2-AMINO-5,6-DIMERCAPTO-7-METHYL-3,7,8A,9-TETRAHYDRO-8-OXA-1,3,9,10-TETRAAZA-ANTHRACEN-4-ONE GUANOSINE DINUCLEOTIDE | C20 H24 N10 O13 P2 S2 | 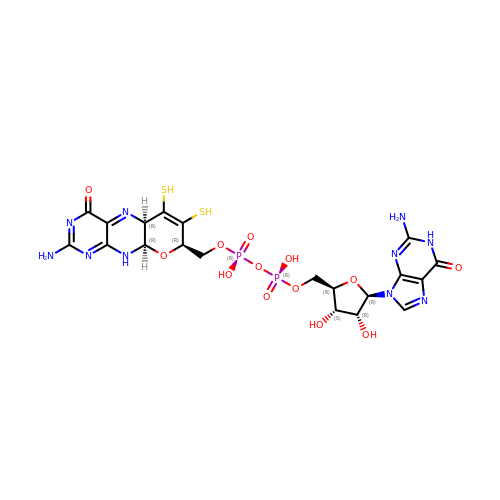SOFMTHSWCZNJTQ-ILXWUORBSA-N>MPKFNHYDLALLNPSFDSPLVDALTELELLRHLRLETDVHPLLFAQLKSIFHMLESLGSARIEGNHTTLADYVESKVEGAEDSTDQLKEIGNIEHAMNFIDEHLHAGEDITEYFVRELHAMTVNGLEREGDKTPGAYRSHGVSIAQSTHLPPEFIHVPAYMQELVGFMNRADAPKYDLMKVALAHHRFGWIHPFGNGNGRTVRLLTYSLLIKYGFNVKTSGRVLNPTAVFCNDRERYYSMLAEADTGAVEGLEQWCLYVLTGISAELKKVDKLSDLHFLNSKVLYPALEYSKGRGVINETESKILKRTISQGTVKTSDLKEVLPGLKPAQITYQIGKLVDRGLLQPVEVGSRIYTAGF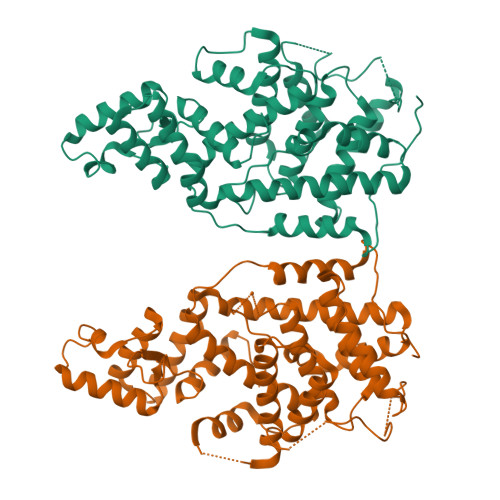SKSDLMRGVIHALRKEGFIPDF[2x]>[3x]MYEAIGHRVEDGVAEITIKLPRHRNA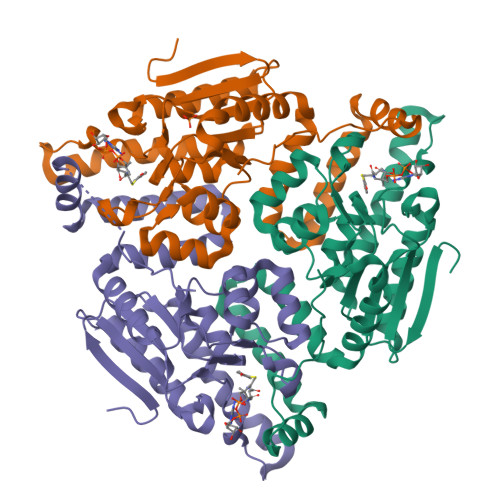LSVKAMQEVTDALNRAEEDDSVGAVMITGAEDAFCAGFYLREIPLDKGVAGVRDHFRIAALWWQQMIHKIIRVKRPVLAAINGVAAGGGLGISLASDMAICADSAKFVCAWHTIGIGNDTATSYSLARIVGMRRAMELMLTNRTLYPEEAKDWGLVSRVYPKDEFREVAWKVARELAAAPTHLQVMAKERFHAGWMQPVEECTEFEIQNVIASVTHPHFMPCLTRFLDGHRADRPQVELPAGV> MAHHHHHHMLKLIVETKTLVQSL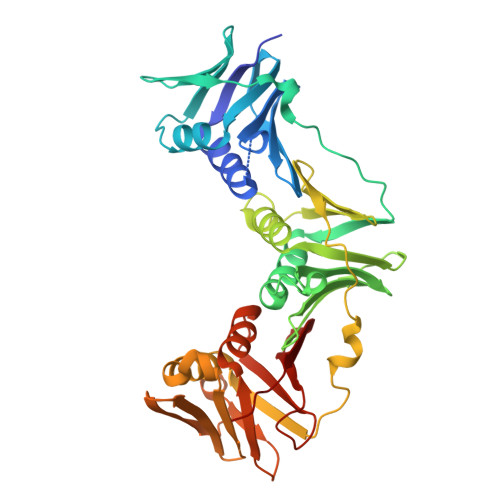GFARSVVEKRNVIPEYANIKLSAKDGNLELSSTNMDLYLSQKIAVQVLSEGEITVSTQTLSDIVRKLPDSELTLTELDIMKLEIKGQNCQFNLFTLPVSSFPAMDSIKPEVSFKISCADFAKIIESTKFSISLDETRYNLNGIYLHIKDKEFFAASTDGHRLSISWITLEEKIKNFGVILPQKSAEEILKIVKDLKNIHEDIEILLSSNKIKFICNENTILLSKLIDGTFPDYSAFIPKSSISKLVINRKIFADSIERIAIITVEKFRAIKLSLSRKTLEISAVGEARGNAKEIITASQDKESFYEYNCDESLVIGFNPQYLEDVLKAVKSNLVELYFSDISASAPVLIKFPQNPKDIFVIMPVKV> RI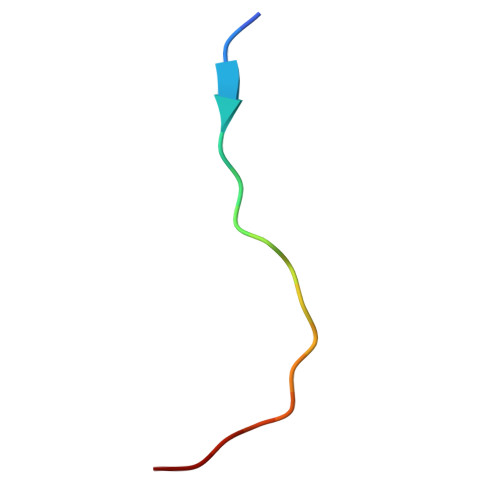QLMTKAARKSAPATG N,N'-dimethyl-N-({3-[4-({trans-3-[2-(tetrahydro-2H-pyran-4-yl)ethoxy]cyclobutyl}oxy)phenyl]-1H-pyrazol-4-yl}methyl)ethane-1,2-diamine 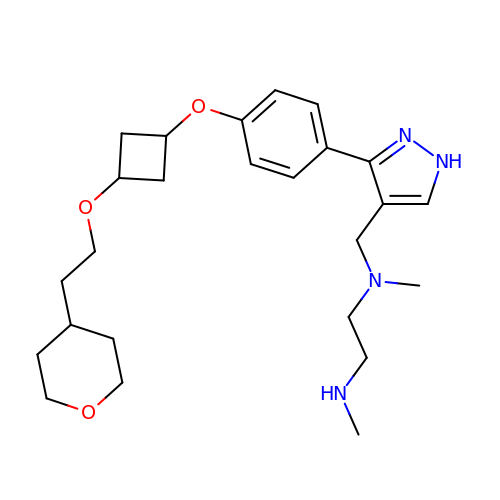| C25 H38 N4 O3 | QMDKVNSQXPVCRD-RQNOJGIXSA-N(S)-2-Amino-5-(2-(methylsulfonyl)acetimidamido)pentanoic acid | C8 H17 N3 O4 S | 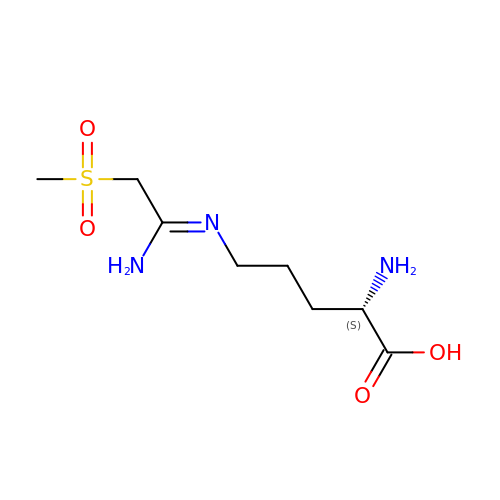ABSOUQYCCCLTCI-LURJTMIESA-N>MKTFIIGISGVTNSGKTTLAKNLQKHLPNCSVISQDDFFKPESEIETDKNGFLQYDVLEALNMEKMMSAISCWMESARHSVVSTDQESAEEIPILIIEGFLLFNYKPLDTIWNRSYFLTIPYEECKRRRSTRVYQPPDSPGYFDGHVWPMYLKYRQEMQDITWEVVYLDGTKSEEDLFLQVY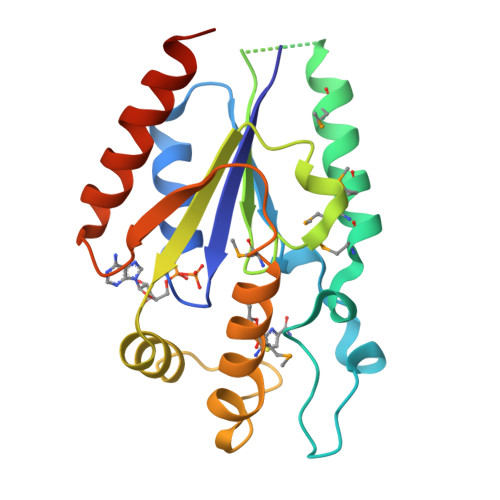EDLIQELAKQKCLQVTA[16x]> MYDSRSSGVHDVAPRDGVDFMYEGPQQVLPGAHPLPLFHPDNSVTRPPVSPYLPSPQRPHPYFTTELPELPHFQTTRPIVYTVGTMKQRIVAPVFDLANNVTHTRELDPFIFGFYPETEEMAKNLSYWLVRCQNFSSKWDYENREIWRKAKKNWPNTGMGMARVGDRKNHAHPWGAHSKPVKPWNLLMPTMDVKTWSKSNRMLVTLKMLQGKLQIVERLTLPEPTQEAYLQLCRTMGWDVRHKGGGALFMDGGSRLTPSSEYDRAFFFGSFFNGRNKLVRPTLLC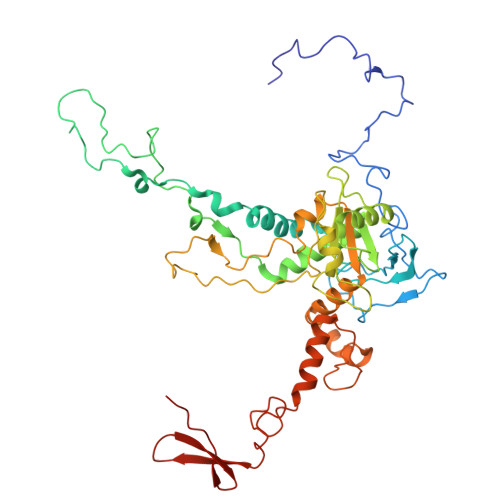DEPYDYNRTSSKARTKGPKGQKNPIPINRFNAYDALTHDTLIITEGALLQLEDEMYTHKLAMLPPHIRAQLPERGFLDSEVLGDVPPALQTVQMEAAARTEEAEQAMYAPYYDNPYHPWQDEGEASYAVDAVEGTVQRYIKSRKTSWAMLS>MMKIVPPKPFFFEAGERAVLLLHGFTGNSADVRMLGRFLESKGYTCHAPIYKGHGVPPEELVHTGPDDWWQDVMNGYEFLKNKGYEKIAVAGLSLGGVFSLKLGYTVPIEGIVTMCAPMYIKSEETSYELVLEYAREYKKREGKSEEQIEQEMEKFKQTPMKTLKALQELKADVRDHLDLIYAPTFVVQARHDEMINPDSANIIYNEIESPVKQIKWYEQSGHVIT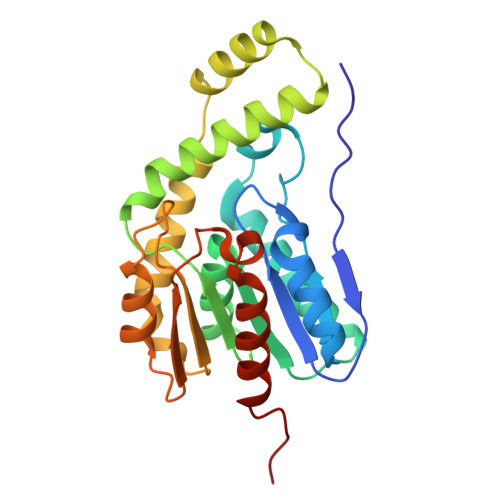LDQEKDQLHEDIYAFLESLDWLEHHHHHH[9x]>[2x]MKIKQALFTAGYSSFYFDDQQAIKNGAGHDGFIYTGDPVTPGFTSVRQAGECVSVQLILENGAVAVGDCAAVQYSGAGGRDPLFLAEHFIPFLNDHIKPLLEGRDVDAFLPNARFFDKLRIDGNLLHTAVRYGLSQALLDATALASGRLKTEVVC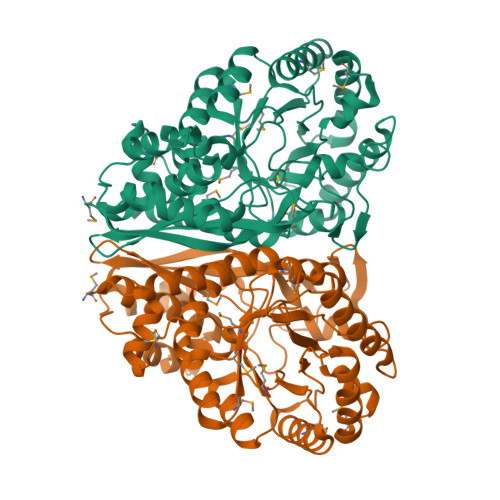DEWQLPCVPEAIPLFGQSGDDRYIAVDKMILKGVDVLPHALINNVEEKLGFKGEKLREYVRWLSDRILSLRSSPRYHPTLHIDVYGTIGLIFDMDPVRCAEYIASLEKEAQGLPLYIEGPVDAGNKPDQIRMLTAITKELTRLGSGVKIVADEWCNTYQDIVDFTDAGSCHMVQIKTPDLGGIHNIVDAVLYCNKHGMEAYQGGTCNETEISARTCVHVALAARPMRMLIKPGMGFDEGLNIVFNEMNRTIALLQTKD>[2x]AHHHHHHHHHHGALEVLFQGPGARASPRTLNLSQLSFHRVDQKEITQLSHLGQGTRTNVYEGRLRVEGSGDPEEGKMDDEDPLVPGRDRGQELRVVLKVLDPSHHDIALAFYETASLMSQVSHTHLAFVHGVCVRGPENIMVTEYVEHGPLDVWLRRERGHVPMAWKMVVAQQLASALSYLENKNLVHGNVCGRNILLARLGLAEGTSPFIKLSDPGVGLGALSREERVERIPWLAP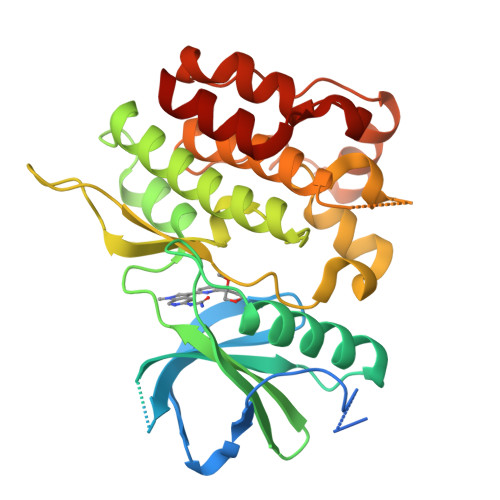ECLPGGANSLSTAMDKWGFGATLLEICFDGEAPLQSRSPSEKEHFYQRQHRLPEPSCPQLATLTSQCLTYEPTQRPSFRTILRDLTRLQ> GHMPPWTARQDSTTGLYAPVTPAGRVLLDRLAAHLPRIRSTAAEHDRDGTFPTDTFDALRKDGLMGATVPAELGGLGVDRLYDVAVALLAVARADASTALALHMQLSRGLTLGYEWRHGDERARTL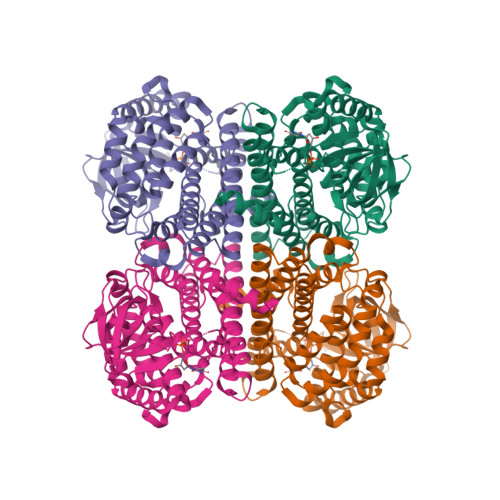AERILRGMVAGDAVVCSGIKDHHTAVTTLRPDGAGGWLLSGRKTLVSMAPVGTHFVINARTDGTDGPPRLASPVVTRDTPGFTVLDNWDGLGMRASGTVDIVFDDCPIPADHVLMRDPVGARNDAVLAGQTVSSVSVLGVYVGVAQAAYDTAVAALERRPEPPQAAALTLVAEIDSRLYALRATAGSALTAADALSADLSGDMDERGRQMMRHFQCAKLAVNRLAPEIVSDCLSLVGGASYTAGHPLARLLRDVQAGRFMQPYAYVDAVDFLSAQALGIERDNNYMSTWAKRSGGNGKSADAAGPRRPTPTSR> GPMAVGPEPLVPSPQPVPEVPSLDPTVLPLYSLGPSGQLAETPAEVFQALEQLGHQAFRPGQERAVMRILSGISTLLVLPTGAGKSLCYQLPALLYSRRSPCLTLVVSPLLSLMDDQVSGLPPCLKAACIHSGMTRKQRESVLQKIRAAQVHVLMLTPEALVGAGGLPPAAQLPPVAFACIDEAHCLSQWSHNFRPCYLRVCKVLRERMGVHCFLGLTATATRRTASDVAQHLAVAEEPDLHGPAPVPTNLHLSVSMDRDTDQALLTLLQGKRFQNLDSIIIYCNRREDTERIAALLRTCLHAAWVPGSGGRAPKTTAEAYHAGMCSRERRRVQRAFMQGQLRVVVATVAFGMGLDRPDVRAVLHLGLPPSFESYVQAVGRAGRDGQPAHCHLFLQPQGEDLRELRRHVHADST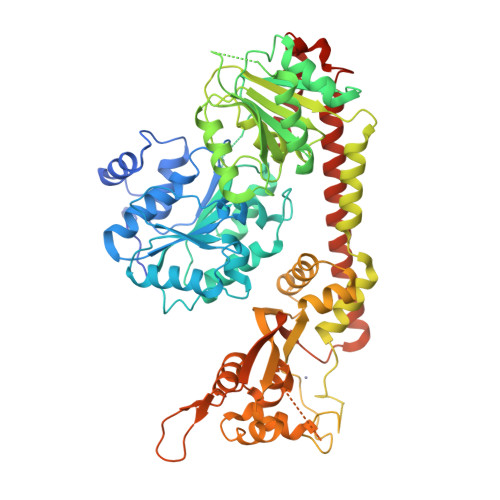DFLAVKRLVQRVFPACTCTCTRPPSEQEGAVGGERPVPKYPPQEAEQLSHQAAPGPRRVCMGHERALPIQLTVQALDMPEEAIETLLCYLELHPHHWLELLATTYTHCRLNCPGGPAQLQALAHRCPPLAVCLAQQLPEDPGQGSSSVEFDMVKLVDSMGWELASVRRALCQLQWDHEPRTGVRRGTGVLVEFSELAFHLRSPGDLTAEEKDQICDFLYGRVQARERQALARLRRTFQAFHSVAFPSCGPCLEQQDEERSTRLKDLLGRYFEEEEGQEP6,7-dimethoxy-2-methyl-~{N}-[(1~{R})-1-[4-[2-(methylaminomethyl)phenyl]thiophen-2-yl]ethyl]quinazolin-4-amine 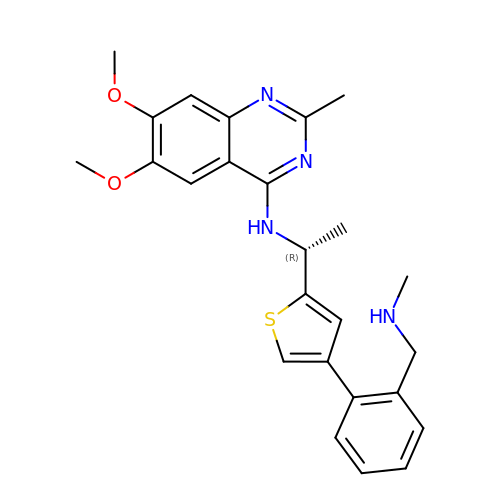| C25 H28 N4 O2 S | WEGLOYDTDILXDA-OAHLLOKOSA-N BENZYL 2-FORMYLPHENYL HYDROGEN PHOSPHATE | C14 H13 O5 P | 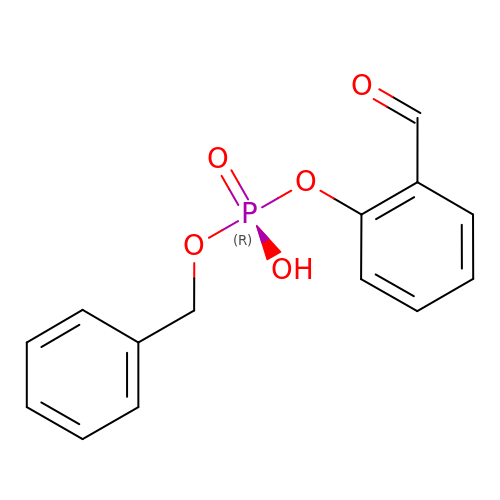PWDTUFYQEUEVQD-UHFFFAOYSA-N>[2x]GHMNSFVGLRVVAKWSSNGYFYSGKITRDVGAGKYKLLFDDGYECDVLGKDILLCDPIPLDTEVTALSEDEYFSAGVVKGHRKESGELYYSIEKEGQRKWYK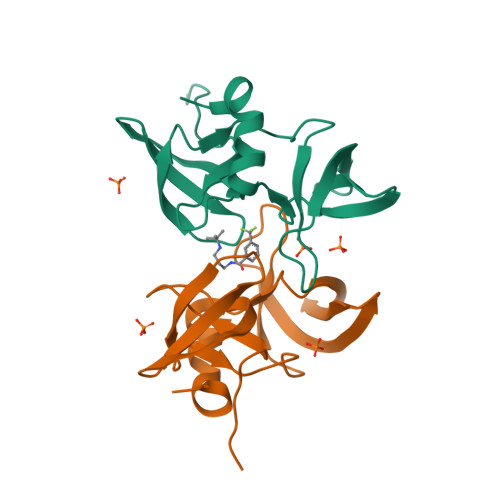RMAVILSLEQGNRLREQYGLG> IARTIVLQESIGKGRFGEVWRGKWRGEEVAVKIFSSREERSWFREAEIYQTVMLRHENILGFIAADNKDNGTWTQLWLVSDYHEHGSLFDYLNRYTVTVEGMIKLALSTASGLAHLHMEIVGTQGKPAIAHRDLKSKNILVKKNGTCCIADLGLAVRHDSATDTIDIAPNHRVGTKRYMAPEVLDDSINMKHFESFKRADIYAMGLVF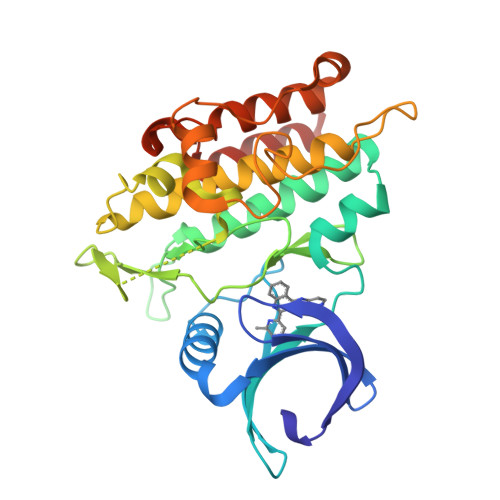WEIARRCSIGGIHEDYQLPYYDLVPSDPSVEEMRKVVCEQKLRPNIPNRWQSCEALRVMAKIMRECWYANGAARLTALRIKKTLSQLSQQEGIKM>APVFAAPVTENYVTVQKDWKNTVKKIQEAIKLKSVTSVEVSYNDKSVSTIDLSGKTKVSELEAEAENLYNLVDSKLSNLDDGDSVTFKVTYNTGFNKRFYSKSELEKIKTQLEKKVVVAKGDGKAAGLAMNENGKAVVADRDLVASDFYNFIISTDTSTGEYILKSEKKGAASLDALNEKYGYAALAIDGTGDFGTVTESYVPAAPTDILKSTKQIDETASFENTGKDIAAMTVKAADPGEDGNIANIKVINAKETTIDVDSKSSTSAEDLAKKYVFDDKDLKAVYDQLNEGDGTTGKYVEKVDGRYQVVLYPEGKRLETKSAS[2x];>TDIENVPAKIVLKADKQKDMKDYIDDLRTYNNSYSNVVTVAGEDRIETAIELSYKYYNSDDDNAVTDIAADNVVLVGSQAIVDGLVASPLASEKHAPLLLTSKDKLDSSVKSEIKRVMDLKTTSGINTSKKVYLAGGVNSISKDVENELKDMGVKVVRLAGDDRYETSLAIADEVGLDNDKAFVVGGTGLADAMSIAPVASQLKDSNGNMDVVDGDATPIVVVDGKAKDINAATEDFLDNAQVDIIGGENSVSKDIEEAIDDATGKEPNRTSGDDRQDTNAEVMKETDYFEKASVENYFVAKDGSTKEDQLVDALAA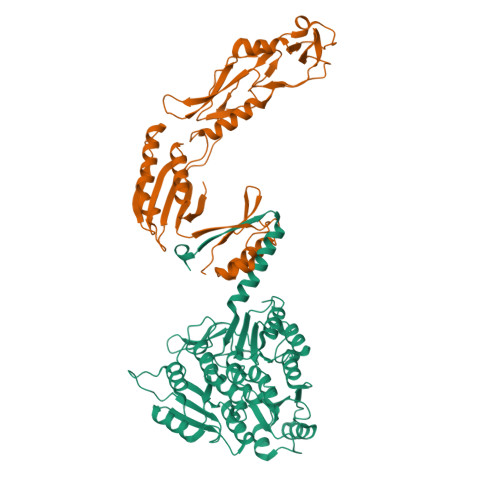APVAANFGATYTKNGSTYTKSGNVSPAPIVLATDTLSGDQNVGVSKSVSDDGGKNLVQVGKGIASSVISKMKDLLDM[2x]Numb functions as an oncosuppressor by inhibiting Notch signaling and stabilizing p53. Numb can also bind to Mdm2, thereby inhibiting its ubiquitin–ligase activity on p53, which physiologically destines the latter to proteasomal degradation. In the four isoforms of Numb, the PTB domain is present as a short version (PTBo in isoform 3 and 4) or a long one (PTBi in isoform 1 and 2), differing for the presence of a stretch of 11 aa coded by Ex3. In this study, we demonstrate that the sequence encoded by Ex3 (11 aa) is responsible for binding to Mdm2 and recapitulates the effects of holo-Numb on p53 and p53-dependent phenotypes.

We determined the crystallographic structure of Numb-PTBi bound to a phosphopeptide (GPpY) derived from a “canonical” PTB-binding adapter protein at 2.8 Å resolution. In the two crystal forms obtained, the canonical PTB fold was extended by the insertion of the Ex3-encoded sequence. The 11-residue Ex3 loop was found to adopt three conformations, all characterized by extension of helix α2 of one or two turns. The crystal structure of Numb-PTBi showed that the Ex3 sequence connects the α2 helix to the β2 strand of the PTBi module adopting several conformations without altering the hydrophobic core of the domain. Ex3 contributed to the formation of a large positively charged patch contributed by lysines 63, 66, 81, 82, and 85 and arginine 64 from Ex3 and flanking regions in the core PTB fold. In addition, the “canonical” phosphopeptide-binding region of the PTB domain was remote and completely distinct from the Ex3-coded region. Indeed, by a variety of approaches, we were able to show that the peptide-binding cleft of PTBi is not involved in the interaction with Mdm2.

>[6x]SRPHQWQTDEEGVRTGKCSFPVKYLGHVEVDESRGMHICEDAVKRLKAERKFFKGFFGKTGKKAVKAVLWVSADGLRVVDEKTKDLIVDQTIEKVSFCAPDRNFDRAFSYICRDGTTRRWICHCFMAVKDTGERLSHAVGCAFAACLERKQKREKE;>[6x]AYIGPYL> MVAITVQGAQLIKRVVERFYPGIAFNINEGACYIYKFSDHIRRIRMKHGTKYRRQAEEIIRNISLRKERLYGIPVLDEVEWKYVFDGQTFQSYAFEVYVNSILPWSELDPEEEFLRNYRVSREMTEVEKFIEFRAKNEMQIYGDIPIKVWCCFINELSAELKHVPLGMQVMADFVNRFDSPFHQGNRDLSNLEDFQVAYTTPLLFEMCCMESILEFNIKMRMREEEISALEFGDMKVDPVGLLREFFILCLPHPKKINNVLRAPYSWFVKMWGVGADPIVVLQSTAGDDRNSKDVFYDKFRTEPNRYKALFRSSFYNESRRMNEEKILEAVKYSQKLGSHDRRLPLFEKMLKTVYTTPFYPHKSSNMILASFLLSIQTITGYGRAWVKNVSTEFDKQLKPNPSNLVQDVSDLTREFFKQAYVEAKERREEIVKPEDLYTSMLRLARNTSSGFSTEIYVKKRFGPRLRDKDLIKINSRIKALVIFTKGHTVFTDEELHKKYNSVELYQTKGSRDVPIKATRTIYSINLSVLVPQLIVTLPLNEYFSRVGGITSPDYKKIGGKVIVGDLEATGSRVMDAADCFRNSADRDIFTIAIDYSEYDTHLTRHNFRTGMLQGIREAMAPYRDLRYEGYTLEQIIDFGYGEGRVANTLWNGKRRLFKTTFDAYIRLDESERDKGSFKVPKGVLPVSSVDVANRIAVDKGFDTLIAATDGSDLALIDTHLSGENSTLIANSMHNMAIGTLMQREVGREQPGVLTFLSEQYVGDDTLFYTKLHTTDTKVFDKVAASIFDTVAKCGHEASPSKTMMTPYSVEKTQTHAKQGCYVPQDRMMIISSERRKDIEDVQGYVRSQVQTMITKVSRGFCHDLAQLILMLKTTFIGAWKMKRTIKEDAMYRDRKFDSNDEDGFTLIQIRNPLALYVPIGWNGYGAHPAALNIVMTEEMYVDSIMISKLDEIMAPIRRIVHDIPPCWNETQGDKRGLISATKMSFFSKMARPAVQAALSDPQIINLVEELPLGEFSPGRISRTMMHSALLKESSARTLLSSGYELEYQKALNSWITQVSMRLGEESGVISTSYAKLFDVYFEGELDGAPHMFPDQNLSPQFYIQKMMIGPRVSSRVRNSYVDRIDVILRKDVVMRGFITANTILNVIEKLGTNHSVGDLVTVFTLMNIETRVAEELAEYMTSEKIRFDALKLLKKGIAGDEFTMSLNVATQDFIDTYLAYPYQLTKTEVDAISLYCTQMIMLRAALGLPKKKMKIVVTDDAKKRYKIRLQRFRTHVPKIKVLKKLIDPNRMTVRNLENQFV;>MAAQNEQRPERIKTTPYLEGDVLSSDSGPLLSVFALQEIMQKVRQVQADYMTATREVDFTVPDVQKILDDIKALAAEQVYKIVKVPSISFRHIVMQSRDRVLRVDTYYEEMSQVGDVITEDEPEKFYSTIIKKVRFIRGKGSFILHDIPTRDHRGMEVAEPEVLGVEFKNVLPVLTAEHRAMIQNALDGSIIENGNVATRDVDVFIGACSEPVYRIYNRLQGYIEAVQLQELRNSIGWLERLGHRKRITYSQEVLTDFRRQDTIWVLALQLPVNPQVVWDVPRSSIANLIMNIATCLPTGEYIAPNPRISSITLTQRITTTGPFAILTGSTPTAQQLNDVRKIYLALMFPGQIILDLKIDPGERMDPAVRMVAGVVGHLLFTAGGRFTNLTQNMARQLDIALNDYLLYMYNTRVQVNYGPTGEPLDFQIGRNQYDCNVFRADFATGTGYNGWATIDVEYREPAPYVHAQRYIRYCGIDSRELINPTTYGIGMTYHCYNEMLRMLVAAGKDSEAAYFRSMLPFHMVRFARINQIINEDLHSVFSLPDDMFNALLPDLIAGAHQNADPVVLDVSWISLWFAFNRSFEPTHRNEMLEVAPLIESVYASELSVMKVDMRHLSLMQRRFPDVLIQARPSHFWKAVLNDSPEAVKAVMNLSHSHNFINIRDMMRWVMLPSLQPSLKLALEEEAWAAANDFEDLMLTDQVYMHRDMLPEPRLDDIERFRQEGFYYTNMLEAPPEIDRVVQYTYEIARLQANMGQFRAALRRIMDDDDWVRFGGVLRTVRVKFYDARPPDDVLQGLPFSYDTNERGGLAYATIKYATETTIFYLIYNVEFSNTPDSLVLINPTYTMTKVFINKRIVERVRVGQILAVLN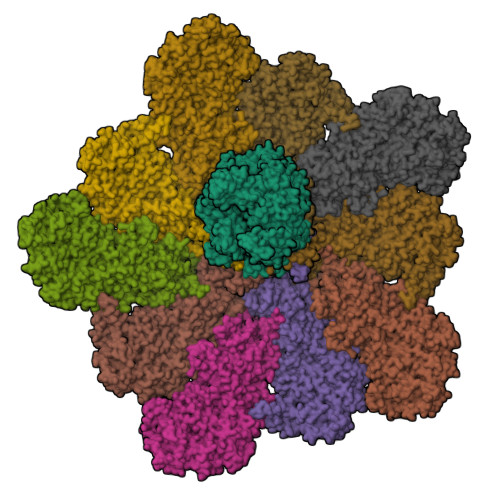RRFVAYKGKMRIMDITQSLKMGTKLAAPTV[10x]(2P)-4-({6-[({[(3aS,4R,7R,10aS)-2,6-diamino-10,10-dihydroxy-3a,4,9,10-tetrahydro-3H,8H-pyrrolo[1,2-c]purin-4-yl]methoxy}carbonyl)amino]hexyl}carbamoyl)-2-{[4aP,9(9a)P]-6-hydroxy-3-oxo-3H-xanthen-9-yl}benzoic acid | C37 H40 N8 O10 | 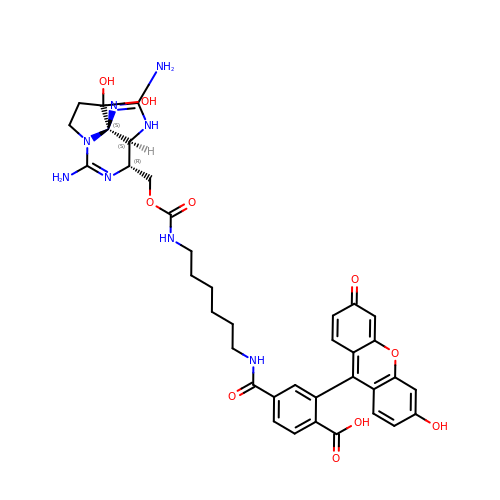QYIDXDKVZLZDCC-FLQVHQRGSA-N>MRNFATLFFMFICLGLSAQVVKEPENMPKEWNQAYEPFRIAGNLYYVGTYDLASYLIVTDKGNILINTGTAESFPIIKANIQKLGFNYKDIKILLLTQAHYDHTGALQDFKTETAAKFYVDKADVDVLRTGGKSDYEMGKYGVTFKPVTPDKTLKDQDKIKLGNITLTLLHHPGHTKGSCSFIFETKDEKRKYRVLIANMPSVIVDKKFSEVTAYPNIQSDYAYTFGVMKKLDFDIWVASHASQFDLHEKRKEGDPYNPQLFMDKQSYFQNLNDLEKSYLNKIKKD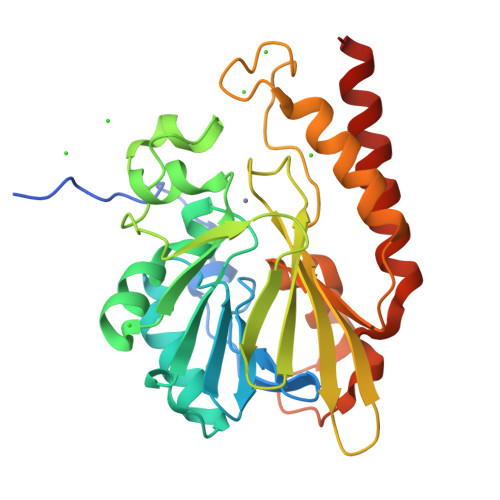SQDK[2x]> GPLGSLKKQYIFQLSSLNPQERIDYCHLIEKLG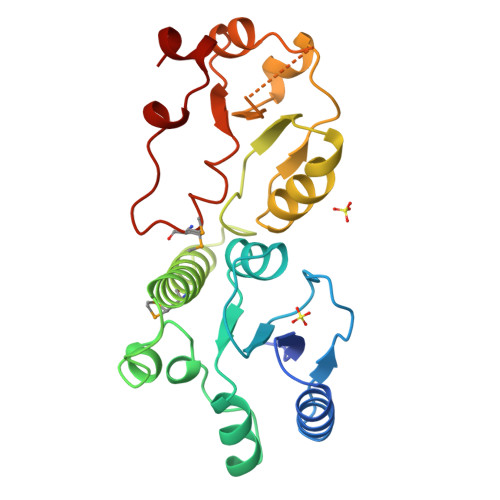GLVIEKQCFDPTCTHIVVGHPLRNEKYLASVAAGKWVLHRSYLEACRTAGHFVQEEDYEWGSSSILDVLTGINVQQRRLALAAMRWRKKIQQRQESGIVEGAFSGWKVILHVDQSREAGFKRLLQSGGAKVLPGHSVPLFKEATHLFSDLNKLKPDDSGVNIAEAAAQNVYCLRTEYIADYLMQESPPHVENYCLPEAISFI4-[2-fluoro-3-(4-oxoquinazolin-3(4H)-yl)phenyl]-7-(2-hydroxypropan-2-yl)-9H-carbazole-1-carboxamide 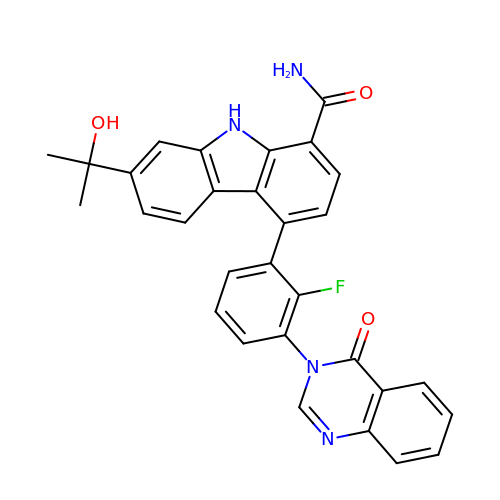| C30 H23 F N4 O3 | WYDRUGJOWSJDHU-UHFFFAOYSA-N(1-HEXADECANOYL-2-TETRADECANOYL-GLYCEROL-3-YL) PHOSPHONYL CHOLINE | C38 H77 N O8 P | 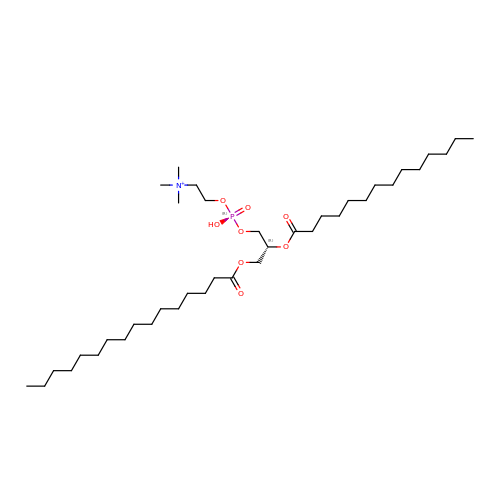UIXXHROAQSBBOV-PSXMRANNSA-O> GNSVTYNTLISGLGKAGRLEEALELFEEMKEKGIVPDVVTYTTLISGLGKAGRLEEALELFEEMKEKGIVPDVVTYNTLISGLGKAGRLEEALELFEEMKEKGIVPDVVTYTTLISGLGKAGRLEEALELFEEMKEKGIVPNVVTYNTLISGLGKAGRLEEALELFEEMKEKGIVPDVVTYTTLISGLGKAGRLEEALELFEEMKEKGI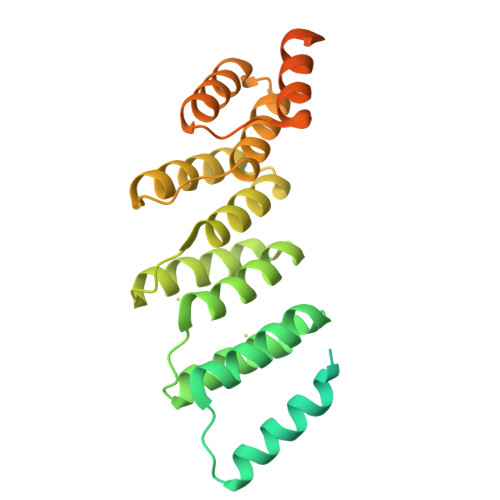VPNVVTYNTLISGLGKAGRLEEALELFEEMKEKGIVPDVVTYTTLISGLGKAGRLEEALELFEEMKEKGIVPNVVTYNTLISGLGKAGCGRALE>[6x]MSGREEIEEAVKEAELKVLAIVLVALRSV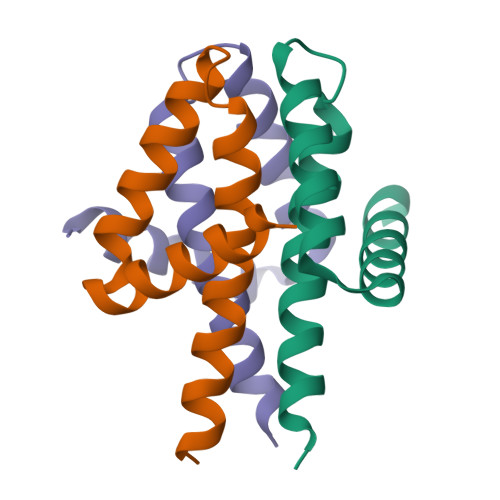SHYEPLSRLYESFLDALKKALSEEELKEVEKEAERIEKKGS PHENYLALANINE-N-SULFONAMIDE 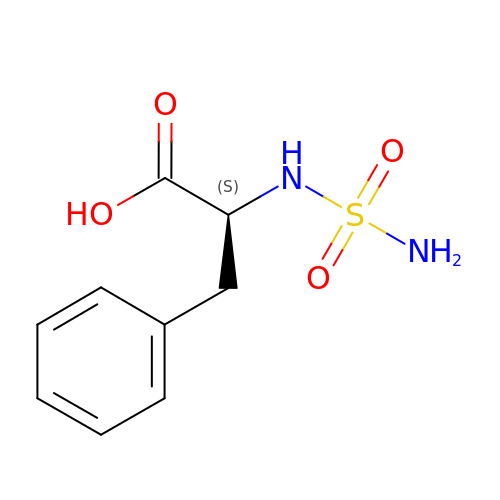| C9 H12 N2 O4 S | PHGMHLLGXKQIDY-QMMMGPOBSA-N>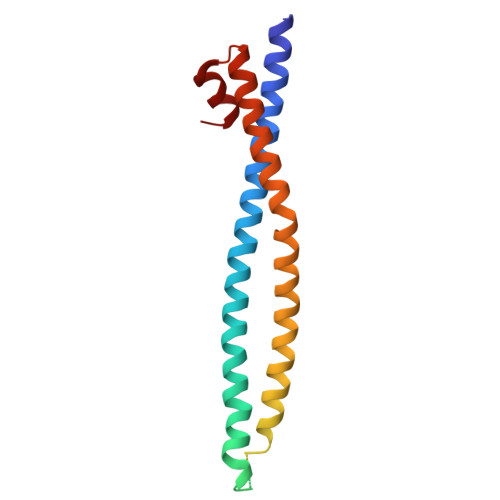 GSKEDSVEAVGAQLKVYHQQYQDKSREYDQLYEEYTRTSQELQMKRTAIEAFNETIKIFEEQGQTQEKSSKEYLERFRREGNEKEMQRILLNSERLKSRIAEIHESRTKLEQQLRAQASDNREIDKRMNSLKPDLMQLRKIRDQYLVWLTQKGARQKKINEWLGI> MSTDVAAAQAQSKIDLTKKKNEEINKKSLEEDDEFEDFPIDTWANGETIKSNAVTQTNIWEENWDDVEVDDDFTNELKA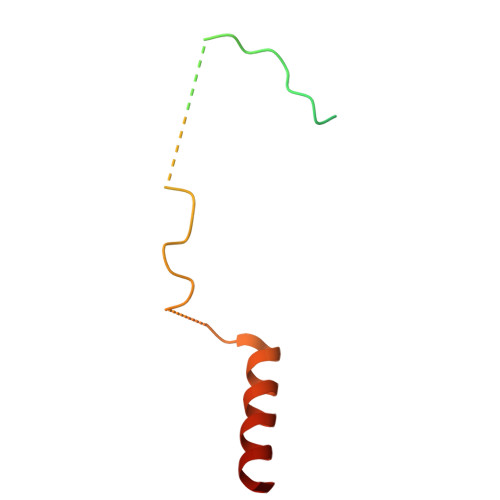ELDRYKRENQ>[2x]ALLLQEAQAGFCRVDGTIDNNHTGFTGSGFANTNNAQGAAVVWAIDATSSGRRTLTIRYANGGTANRNGSLVIN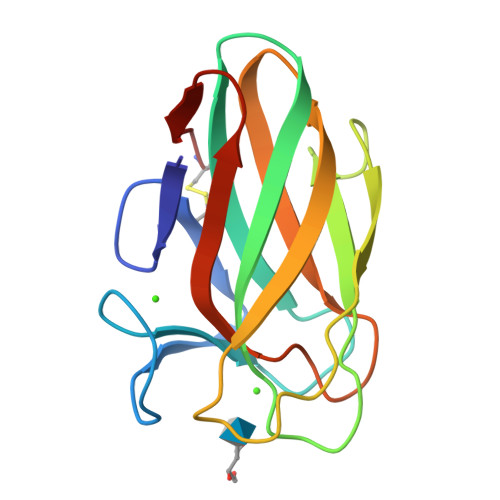GGSNGNYTVSLPTTGAWTTWQTATIDVDLVQGNNIVQLSATTAEGLPNIDSLSVVGGTVRAGNCG> MANELTWHDVLAEEKQQPHFLNTLQTVASERQSGVTIYPPQKDVFNAFRFTELGDVKVVILGQDPYHGPGQAHGLAFSVRPGIAIPPSLLNMYKELENTIPGFTRPNHGYLESWARQGVLLLNTVLTVRAGQ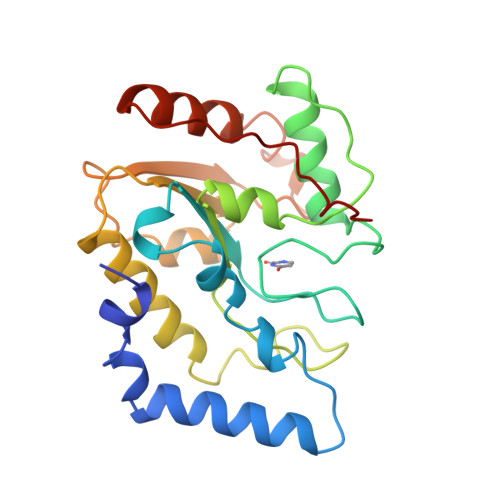AHSHASLGWETFTDKVISLINQHREGVVFLLWGSHAQKKGAIIDKQRHHVLKAPHPSPLSAHRGFFGCNHFVLANQWLEQHGETPIDWMPVLPAESE> MSLNNITFCVSQDLDVPLKVKIKSLEGHKPLLKPSQKILNPELMLIGSNVFPSSDLIVSLQVFDKERNRNLTLPIYTPYIPFRNSRTWDYWLTLPIR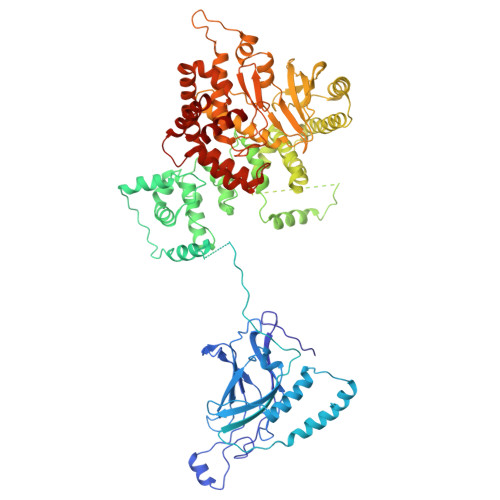IKQLTFSSHLRIILWEYNGSKQIPFFNLETSIFNLKDCTLKRGFESLKFRYDVIDHCEVVTDNKDQENLNKYFQGEFTRLPWLDEITISKLRKQRENRTWPQGTFVLNLEFPMLELPVVFIEREIMNTQMNIPTLKNNPGLSTDLREPNRNDPQIKISLGDKYHSTLKFYDPDQPNNDPIEEKYRRLERASKNANLDKQVKPDIKKRDYLNKIINYPPGTKLTAHEKGSIWKYRYYLMNNKKALTKLLQSTNLREESERVEVLELMDSWAEIDIDDALELLGSTFKNLSVRSYAVNRLKKASDKELELYLLQLVEAVCFENLSTFSDKSNSEFTIVDAVSSQKLSGDSMLLSTSHANQKLLKSISSESETSGTESLPIVISPLAEFLIRRALVNPRLGSFFYWYLKSESEDKPYLDQILSSFWSRLDKKSRNILNDQVRLINVLRECCETIKRLKDTTAKKMELLVHLLETKVRPLVKVRPIALPLDPDVLICDVCPETSKVFKSSLSPLKITFKTTLNQPYHLMFKVGDDLRQDQLVVQIISLMNELLKNENVDLKLTPYKILATGPQEGAIEFIPNDTLASILSKYHGILGYLKLHYPDENATLGVQGWVLDNFVKSCAGYCVITYILGVGDRHLDNLLVTPDGHFFHADFGYILGQDPKPFPPLMKLPPQIIEAFGGAESSNYDKFRSYCFVAYSILRRNAGLILNLFELMKTSNIPDIRIDPNGAILRVRERFNLNMSEEDATVHFQNLINDSVNALLPIVIDHLHNLAQYWRT> GM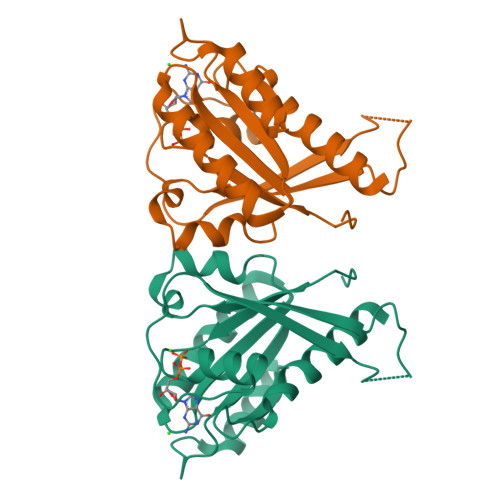EKKSSYKTVLLGESSVGKSSIVLRLTKDTFHENTNTTIGASFCTYVVNLNDINIKNNSNNEKNNNINSINDDNNVIITNQHNNYNENLCNIKFDIWDTAGQERYASIVPLYYRGATCAIVVFDISNSNTLDRAKTWVNQLKISSNYIIILVANKIDKNKFQVDILEVQKYAQDNNLLFIQTSAKTGTNIKNIFYMLAEEIYKNIIN> IESIIKTATDTVK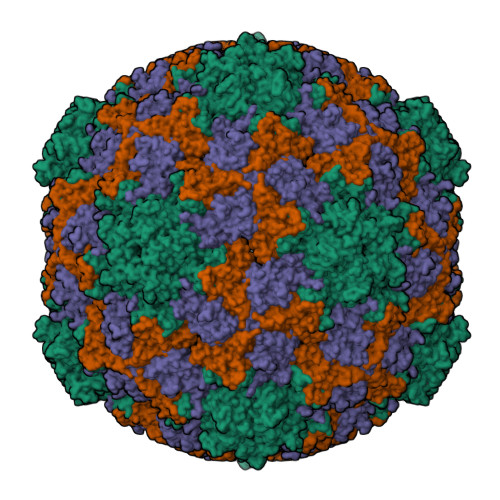SEINAELGVVPSLNAVETGASSNTEPEEAIQTRTVINQHGVSETLVENFLSRAALVSKRSFEYKNHTSSEARTDKNFYKWTINTKSFVQLRRKLELFTYLRFDAEITILTTVAVGSNNSTYMGLPDLTLQAMFVPTGALTPEKQDSFHWQSGSNASVFFKVSDPPARMTIPFMCINSAYSVFYDGFAGFEKNGLYGINPADTIGNLCVRIVNEHQPIGFTVTVRVYMKPKHIKAWAPRPPRTLPYMSIANANYKGKERAPNALNAIIGNRESVKTMPHDIRLV;> SPSAEACGYSDRVLQLKLGNSAIVTQEAANYCCAYGEWPNYLPDHEAVAIDKPTQPETATDRFYTLKSVKWETESTGWWWKLPDALNNIGMFGQNVQHHYLYRSGFLIHVQCNATKFHQGALLVVAIPEHQRGAHNTTTSPGFDDIMKGEEGGTFNHPYVLDDGTSLACATIFPHQWINLRTNNSATIVLPWMNAAPMDFPLRHNQWTLAIIPVVPLGTRTVSSMVPITVSIAPMCCEFNGLRHAITQ;> GVPTYLLPGSGQFLTTDDHSSAPVLPCFNPTPEMHIPGQVRNMLEVIQVESMMEINNTENAVGMQRLKVDISVLTDVDQLLFNIPLDIQLDGPLRNTLVGNISRYYTHWSGSLEMTFMFCGSFMATGKLILCYTPPGGSCPTTRETAMLGTHIVWDFGLQSSVTLVIPWISGSHYRMFNNDAKSTNANVGYVTCFMQTNLIVPSESSNTCSLIGFVAAKDDFSLRLMRDSPDIGQLEHLHEAEAAYQ>[2x]MSEDLRVGLFPVRYLVGTGLPGAPQLVLDLMVDTVDHSVVGRAAVSQAVSPPLNFHADVWG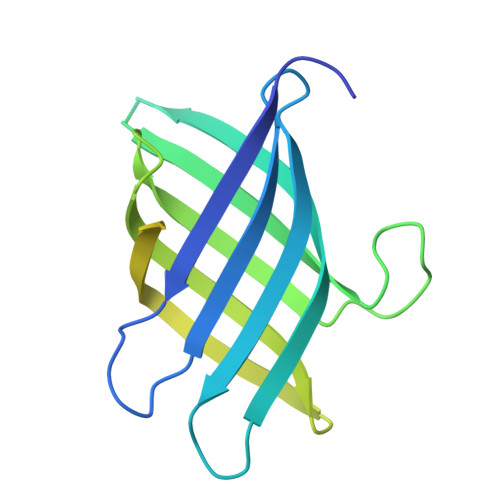SYVFRLGPPPRRDGSGAIVQISLQGNQGGPQSNSMITFYGELLLKGDGKTGVASYRYYSNGSWHEVENVPVKADPELVPIEPGPVIGQSSMSAIGSAAMYGVAIQSAAASGDLAHMRTLSAYARQQLESRDEIAAALSELKAEIAKLESRQHHHHHH> MVAEKETLSLNKCPDKMPKRTKLLAQQPLPVHQPHSLVSEGFTVKAMMKNSVVRGPPAAGAFKERPTKPTAFRKFYERGDFPIALEHDSKGNKIAWKVEI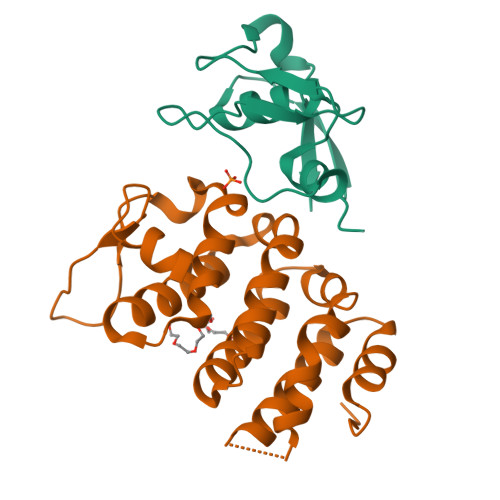EKLDYHHYLPLFFDGLCEMTFPYEFFARQGIHDMLEHGGNKILPVLPQLIIPIKNALNLRNRQVICVTLKVLQHLVVSAEMVGKALVPYYRQILPVLNIFKNMNVNSGDGIDYSQQKRENIGDLIQETLEAFERYGGENAFINIKYVVPTYESCLLN;> GPLGSMASSDVKPKSVSHAKKWSEEIENLYRFQQAGYRDETEYRQVKQVSMVDRWPETGYVKKLQRRDNTFYYYNKQRECDDKEVHKVKIYAY>[2x]YVEGQRKRRNTIHEFKKSAKTTLIKIDPALKIKTKKVNTADQCANRCTRNKGLP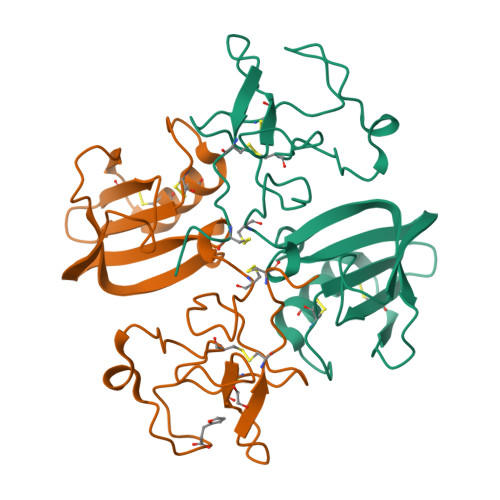FTCKAFVFDKARKQCLWFPFNSMSSGVKKEFGHEFDLYENKDYIRNCIIGKGRSYKGTVSITKSGIKCQPWSSMIPHEHSFLPSSYRGKDLQENYCRNPRGEEGGPWCFTSNPEVRYEVCDIPQCSEVE> MIAEELLRAGRLDDALKALQEQVRSQPSNATLRIFLFQLLAVMGQWARAQNQLKVVGELDASALPMVQTYSTAIDCEALRREVFAGRLTPVILGQPAEWIAPLLQALSLDAEGHGEAAQALREQAFDAAPAVPGRIGEAPFAWLADA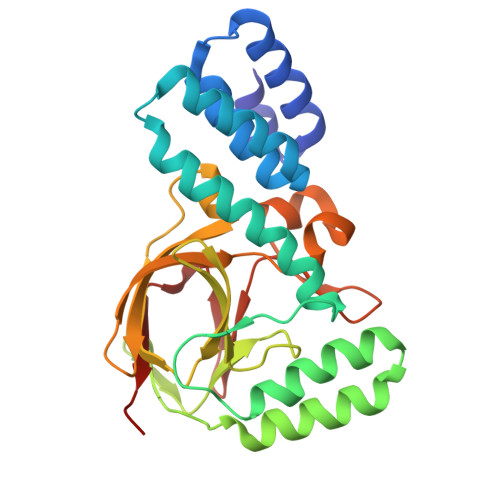DTRLGPVLEVIVNGRYAWLPMSNLRSLKVEAPSDLRDLVWLPAELTLANGGATVALLPARYAETVEHGDDAARLGRKTEWLDSGLPVGQRLFVTDAGETALFDLRELDFEPTDA>[2x]MDPYSETSDLVDISRFDTHGLGANYKLRRHKFEHLADTGCHKARSDWVKY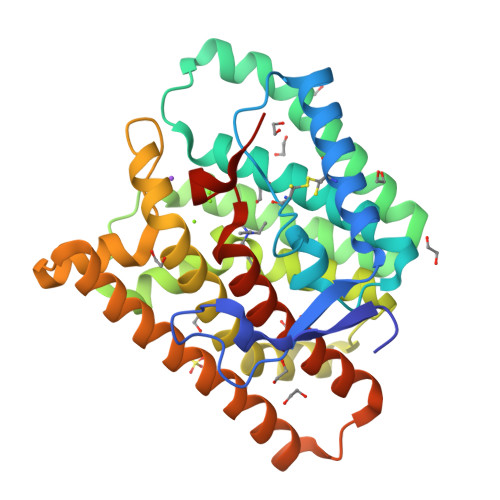IGPLTEFGGCNHINGNFSAVVLPLCRPDRLELIAYVLEFAFLHDSVLESENTSPESEVQAEAGLRLLYERCISRLLQTDEVCAKKIAKTWKDAINTTTKDKNVDFQSIEDYLEFRMIDTGAPFVEALMLFGLGMSLSPQEDDALGHVIRPCFAALALTNDYFSFDREIEEVDTSTLINSVAIVMRIQSLDIPTAKTIINETIQKYEREFLRRIDEYKQHKGPISNKIEQYMEAMTYQISGNLVWSLNCPRYNPDYRYGLEACQHEG N-[4-METHYL-3-[[4-(3-PYRIDINYL)-2-PYRIMIDINYL]AMINO]PHENYL]-3-PYRIDINECARBOXAMIDE 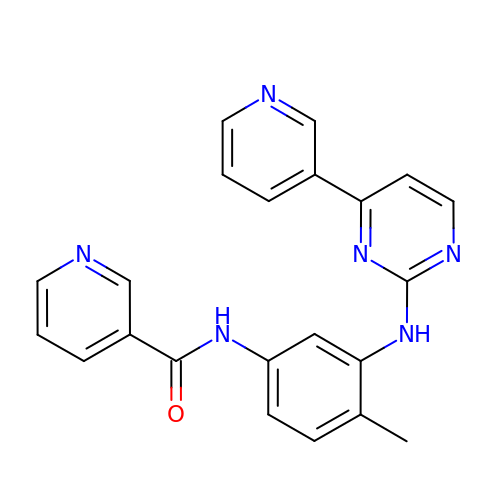| C22 H18 N6 O | YWQVBESSYLICRX-UHFFFAOYSA-N>[2x]MNPHSIVKIISLCFFWIPICLVCKIREEKGTYKNLEEALRNPDKVFVLKM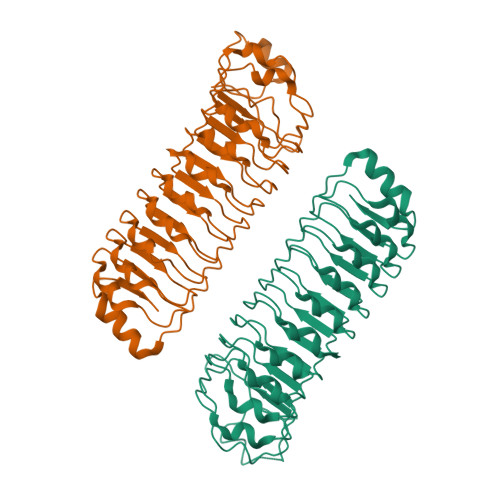KGTERTKLVTLSREIVRFQNLKELDLEGNQLKEFPKEIGNLKNLRKLDLSENPLMFFPKEITNLESLEELNISGTELTIIPKEIGNMNGLLRLYLDENPFSELPKEIGNLKNVLRLYLSNTFLKTLPKEIGEMQSLEELNATGTSLSKLPKEIGNLKNLSNLNLSRTELTTLPKEIGGLRNVRLLYLETSRLELLPKEIGNLRNLEELYLYQNRITELPKEIGNLQNLKLLHLNGNLLETLPKEIGNLKNLKLLHLSKNRFSPEERKRIRQLLPNCEIYF>TRDQNGTWEMESNENFEGYMKALDIDFATRKIAVRLTQTLVIDQDGDNFKTKTTSTFRNWDVDFTVGVEFDEYTKSLDNRHVKALVTWEGDVLVCVQKGEKENRGWKKWIEGDKLYLELT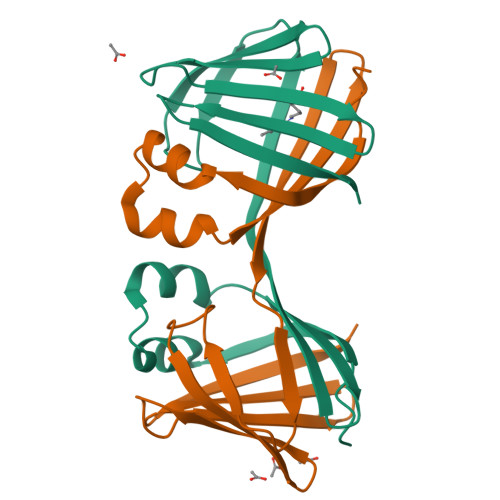CGDQVCRQVFKKK[2x]>[2x]MGIDTGTSNLVAVEPGAIREDTPAGSVIQYSDYEIDYSSPFAGGVAWIEGEYLPAEDAKISIFDTGFGHSDLTYTVAHVWHGNIFRLGDHLDRLLDGARKLRLDSGYTKDELADITKKCVSLSQLRESFVNLTITRGYGKRKGEKDLSKLTHQVYIYAIPYLWAFPPAEQIFGTTAVVPRHVRRAGRNTVDPTIKNYQWGDLTAASFEAKDRGARTAILMDADNCVAEGPGFNV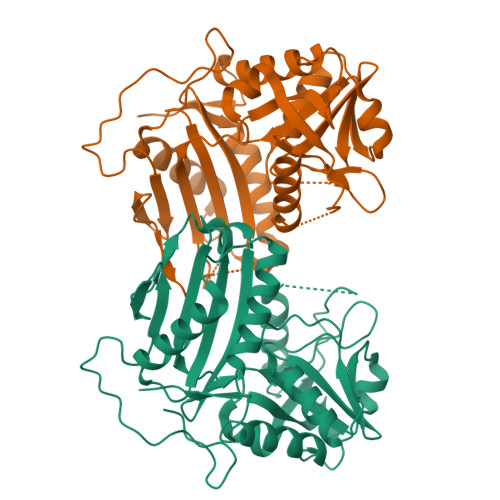CIVKDGKLASPSRNALPGITRKTVFEIAGAMGIEAALRDVTSHELYDADEIMAVTTAGGVTPINTLDGVPIGDGEPGPVTVAIRDRFWALMDEPGPLIEAIQY>[2x]ATSSPNVQVYTYKLIKEGESNVL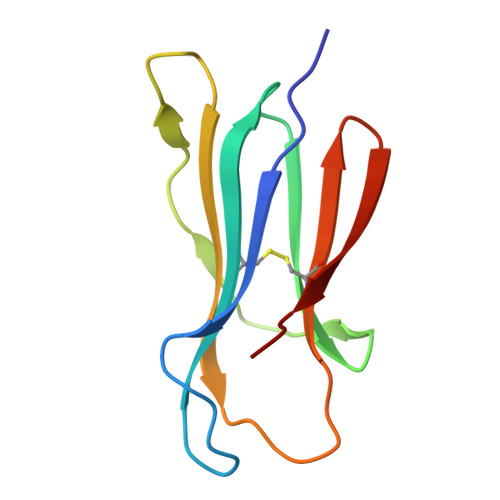LCHAKDFSPPNIKLELLENGRIIPNTTQSDLSFESDWSFKLTRYVEFTPQSGYKYSCMVTHNGDSKEIQLDRY> GSFVEMVDNLRGKSGQGYYVEMTVGSPPQTLNILVDTGSSNFAVGAAPHPFLHRYYQRQLSSTYRDLRKGVYVPYTQGKWEGELGTDLVSIPHGPNVTVRANIAAITESDKFFINGSNWEGILGLAYAEI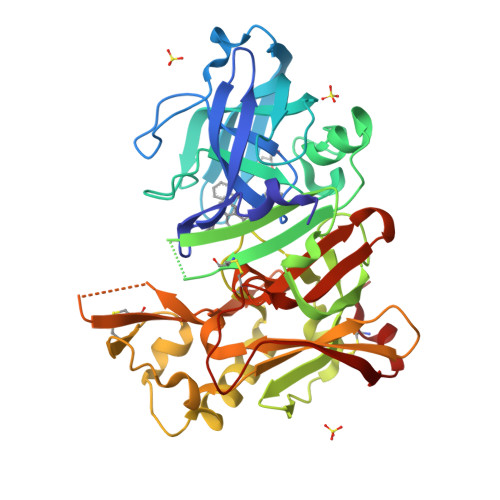ARPDDSLEPFFDSLVKQTHVPNLFSLQLCGAGFPLNQSEVLASVGGSMIIGGIDHSLYTGSLWYTPIRREWYYEVIIVRVEINGQDLKMDCKEYNYDKSIVDSGTTNLRLPKKVFEAAVKSIKAASSTEKFPDGFWLGEQLVCWQAGTTPWNIFPVISLYLMGEVTNQSFRITILPQQYLRPVEDVATSQDDCYKFAISQSSTGTVMGAVIMEGFYVVFDRARKRIGFAVSACHVHDEFRTAAVEGPFVTLDMEDCGYN>MRGSHHHHHHGLVPRGSMQNPRTVSDTKRAFYAAHTRPIHSIYRRFIEELLVEIHLLRVNVDFRYSPLFALGVVTAFDQFMEGYQPEGDRDRIFHALCVAEEMNPQQLKEDAASWQQYQGRPLSQILDELNSGQPSAPLNSLNHTGKYSRLHAVGLYAFLQELAGEVTIHLNETLDQLAPVIPLPIEKVKRDLELYRSNLDKINQARSLMKELVEQERKRRAQQTSAPPAVDASSDAPA[7x]

Here we show that Psb29 in Synechocystis 6803, like THF1 in Arabidopsis, is important for normal accumulation of the FtsH heterocomplex involved in PSII repair. To gain further insights into Psb29, we have determined the crystal structure of Psb29 encoded by Thermosynechococcus elongatus, a thermophilic cyanobacterium widely used to study structural aspects of PSII assembly and repair. Each Psb29 subunit consists of 9 alpha helices. A search using PDBeFOLD found no known structures with greater than 70% similarity, indicating that the specific fold is novel.

For preparations in the presence of protease inhibitor, the only crystals obtained were of needle morphology in P6322, which diffracted very weakly. The P6322 form was soaked overnight in 1 mM 4-(Chloromercuri)benzensulfonic acid sodium salt (Jena Bioscience), but this was not used for phase determination. The B-P21,I222 and P6322 crystal forms were solved by molecular replacement with Phaser using the A-P21 structure as a model. The most complete structure consisting of residues 4 to 206 of the predicted 222 residues of Psb29 was obtained from P6322 needle-shaped crystals containing seven copies of Psb29 in the asymmetric unit, which form a continuous cylindrical shell of protein in the crystal, with the C-terminus of the protein forming a helix extending from the compact protein fold into the middle of the cylindrical protein shell. A striking feature of Psb29 is the presence of a long alpha helix at the C-terminus extending from the globular protein domain. The first 3 and last 16 residues could not be identified in the most complete crystal structure, possibly because of structural flexibility or because of some proteolytic degradation. In the B-P21 crystal form, the new carboxy terminus at residue Ala189 is clearly visible in the electron density. It is likely that proteolytic cleavage of the C-terminal helix allows more compact higher resolution crystal lattices to form, as there is insufficient space in these lattices to accommodate the C-terminal helix observed in the P6322 crystal form.>GSMGKDEALEKDLNDVSKEINLMLSTYAKLLSERAAVDASYIDEIDELFKEANAIENALIQKREELRQRFTAIANTLHR[4x]

Meiosis protein TEX12 is an essential component of the synaptonemal complex (SC), which mediates homologous chromosome synapsis. It is also recruited to centrosomes in meiosis, and aberrantly in certain cancers, leading to centrosome dysfunction. Within the SC, TEX12 forms an intertwined complex with SYCE2 that undergoes fibrous assembly, driven by TEX12’s C-terminal tip. TEX12 undergoes conformational change upon C-terminal tip mutations, indicating that the sequence responsible for driving SYCE2-TEX12 assembly within the SC also controls the oligomeric state and conformation of isolated TEX12.

Our crystal structure of an FFV dimer in a helical conformation demonstrates a unique, phase-shifted anti-parallel conformation. Owing to the phase shift, the centre of this alternative FFV dimer lacks the R78-D82 hinge present within ΔCtip and FFV dimer structures. Instead, its centre is characterised by a stacking interaction of central Y85 residues. Importantly, TEX12’s Ctip sequences directly contribute to the dimeric coiled-coil, while 10 amino-acids at the TEX12’s N-termini were not visible in electron density. In the crystal lattice, hydrophobic surfaces of coiled-coil ends (formed by Ctip and the N-terminus) mediate dimer-of-dimer interactions between obliquely-oriented molecules. These interactions are recursive, generating a right-handed helix of FFV dimers that is continuous throughout the lattice, and is intertwined with another FFV helix in a double-helical arrangement. Thus, while we cannot exclude the possibility of the helical dimer forming in some context in vivo, it does not explain any solution state of TEX12, and likely constitutes an artefact of crystallisation.> GAMTFTRYSRLRVIAEIRHGDIFHSANIVSSIEFSDRDDELFATAGVSRCIKVFDFSSVVNEPADMQCPIVEMSTRSKLSCLSWNKHEKNHIASSDYEGIVTVWDVTTRQSLMEYEEHEKRAWSVDFSRTEPSMLVSGSDDCKVKVWCTRQEASVINIDMKANIC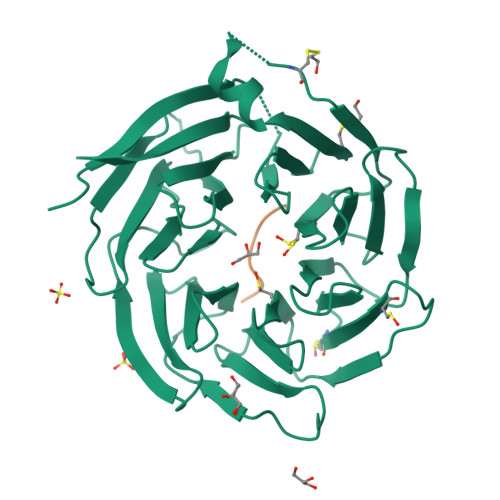CVKYNPGSSNYIAVGSADHHIHYYDLRNISQPLHVFSGHKKAVSYVKFLSNNELASASTDSTLRLWDVKDNLPVRTFRGHTNEKNFVGLTVNSEYLACGSETNEVYVYHKEITRPVTSHRFGSPDMDDAEEEAGSYFISAVCWKSDSPTMLTANSQGTIKVLVLAA;> XRYAVVPDE>[2x]GPLGSEILNNIILNLRYKDNNLIDLSGYGAKVEVYDGVELNDKNQFKLTSSANSKIRVTQNQNIIFNSVFLDFSVSFWIRIPKYKNDGIQNYIHNEYTIINCMKNNSGWKISIRGNRIIWTLIDINGKTKSVFFEYNIREDISEYINRWFFVTITNNLNNAKIYINGKLESNTDIKDIREVIANGEIIFKLDGDIDRTQFIWMKYFSIFNTELSQSNIEERYKIQSYSEYLKDFWGNPLMYNKEYY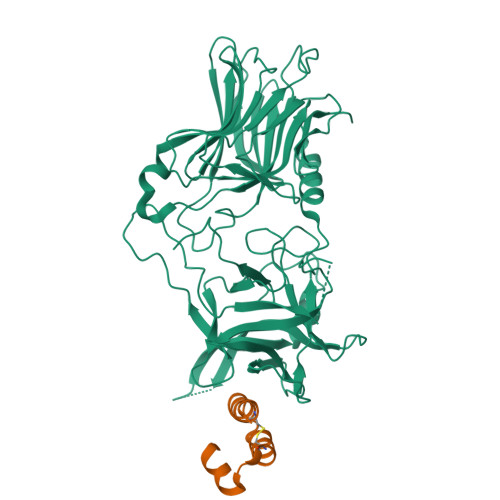MFNAGNKNSYIKLKKDSPVGEILTRSKYNQNSKYINYRDLYIGEKFIIRRKSNSQSINDDIVRKEDYIYLDFFNLNQEWRVYTYKYFKKEEEKLFLAPISDSDEFYNTIQIKEYDEQPTYSCQLLFKKDEESTDEIGLIGIHRFYESGIVFEEYKDYFCISKWYLKEVKRKPYNLKLGCNWQFIPKDEGWTE;>[2x]PDMFCALKIKFFLEIGDEDAARKAAKKCGYSEEQAERIIKKNL>MITDEHIELFLAQAHRYGDAKLMLCSSGNLSWRIGEEALISGTGSWVPTLAKEKVSICNIASGTPTNGVKPSMESTFHLGVLRERPDVNVVLHFQSEYATAISCMKNKPTNFNVTAEIPCHVGSEIPVIPYYRPGSPELAKAVVEAMLKHNS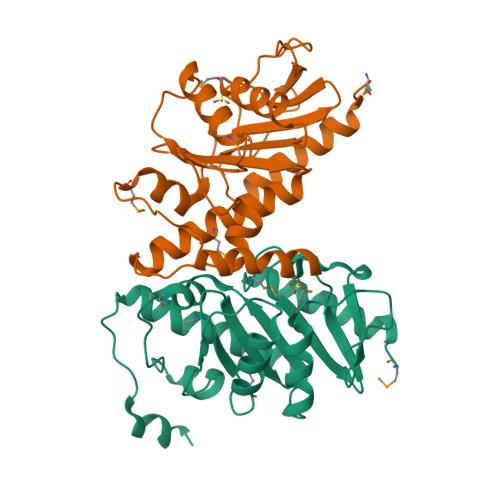VLLTNHGQVVCGKDFDQVYERATFFEMACRIIVQSGGDYSVLTPEEIEDLEIYVLGKKTK[2x]>[3x]GSMRKL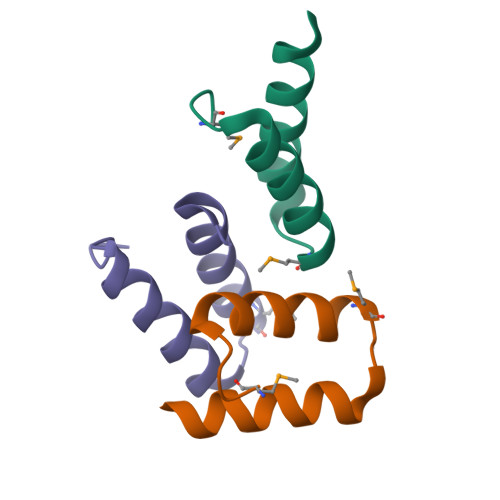SDELLIESYFKATEMNLNRDFIELIENEIKRRSLGHIISVSS>[2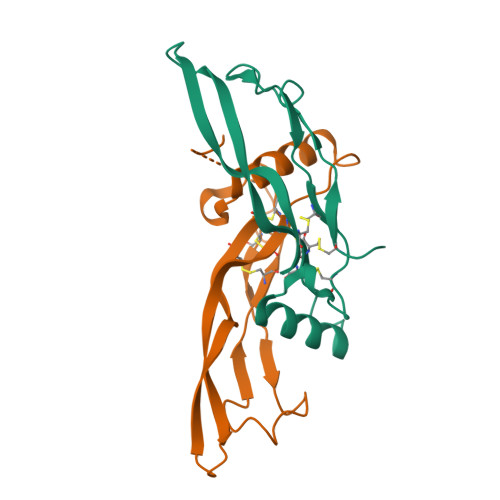x]APLATRQGKRPSKNLKAECSRKALHVNFKDMGWDDWIIAPLEYEAFHCEGLCEFPLRSHLEPTNHAVIQTLMNSMDPESTPPTCCVPTRLSPISILFIDSANNVVYKQYEDMVVESCGCR>[2x]MNMKNKFSFLLLLLTIYGFAQEKNKQPEGFPFILPKEKPNRPLSAAMQRNYDNYMAPRPENNELYTQFKYTELKGFDYNGHDGTISRRDPSKVIYENGKYYVWYTYRNTPTPPQGAKNSNDTIPSADWDLAEIWYATSKDGFTWEEQGVAVPRPPKPNVGWRSVTTTDILKWKGKFY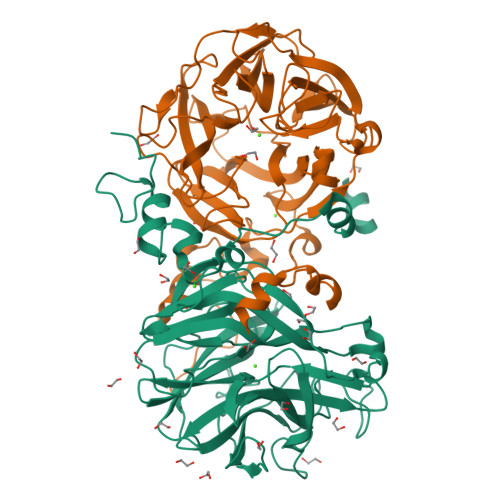LYYQGFMEASGTRGDDCPVAVSYADSPDGPWTPHTEVVIPNGKKGEWDQYSIHDPYPIVYKDKIYLYYKSDFDGDPNLVRMQGLAIADNPLGPFKKSPLNPVINSGHETTLFPFKEGMAALVIRDGTEHNTVQYAEDGVNFNIASIVEFMPNAAGPYVADAFTNTKYGRGISWGISHFTNATTWDQNHAVLARFDCDLSLDVDDPHMKRLGTYFKPEFYYQMGLSKKQRERIEKQPK>[3x]METSDIQIFYQEDPECQNLSENSCPPSEVSDTNLYSPFKPRNYQLELALPAMKGKNTIICAPTGCGKTFVSLLICEHHLKKFPQGQKGKVVFFANQIPVYEQQKSVFSKYFERHGYRVTGISGATAENVPVEQIVENNDI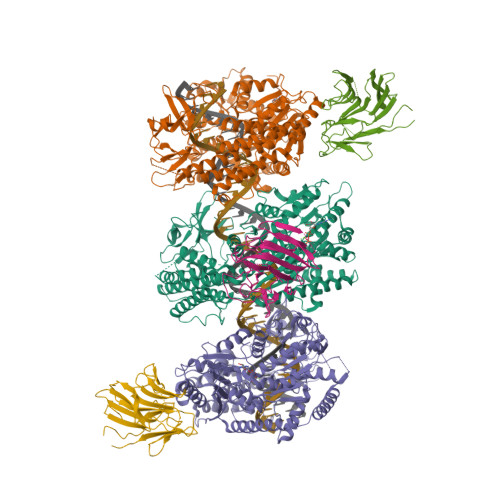IILTPQILVNNLKKGTIPSLSIFTLMIFDECHNTSKQHPYNMIMFNYLDQKLGGSSGPLPQVIGLTASVGVGDAKNTDEALDYICKLCASLDASVIATVKHNLEELEQVVYKPQKFFRKVESRISDKFKYIIAQLMRDTESLAKRICKDLENLSQIQNREFGTQKYEQWIVTVQKACMVFQMPDKDEESRICKALFLYTSHLRKYNDALIISEHARMKDALDYLKDFFSNVRAAGFDEIEQDLTQRFEEKLQELESVSRDPSNENPKLEDLCFILQEEYHLNPETITILFVKTRALVDALKNWIEGNPKLSFLKPGILTGRGKTNQNTGMTLPAQKCILDAFKASGDHNILIATSVADEGIDIAQCNLVILYEYVGNVIKMIQTRGRGRARGSKCFLLTSNAGVIEKEQINMYKEKMMNDSILRLQTWDEAVFREKILHIQTHEKFIRDSQEKPKPVPDKENKKLLCRKCKALACYTADVRVIEECHYTVLGDAFKECFVSRPHPKPKQFSSFEKRAKIFCARQNCSHDWGIHVKYKTFEIPVIKIESFVVEDIATGVQTLYSKWKDFHFEKIPFDPAEMSK;>RRASRFAQWAIHPTFNLKSLSCSLEVSKDSRTVTVSHRPQPYRWSCERFSTSQVLCSQALSSGKHYWEVDTRNCSHWAVGVASWEMSRDQVLGRTMDSCCVEWKGTSQLSAWHMVKETVLGSDRPGVVGIWLNLEEGKLAFYSVDNQEKLLYECTISASSPLYPAFWLYGLHPGNYLIIKQVKV[3x]> QRDDFHWEEYLKETGSISAPSECFRQSQIPPVNDF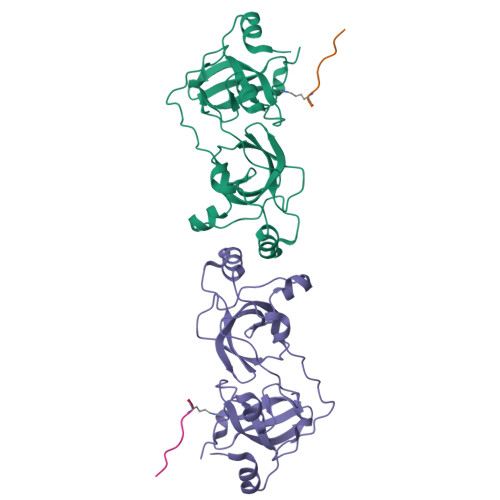KVGMKLEARDPRNATSVCIATVIGITGARLRLRLDGSDNRNDFWRLVDSPDIQPVGTCEKEGDLLQPPLGYQMNTSSWPMFLLETLNGSEMASATLFKKEPPKPPLNNFKVGMKLEAIDKKNPYLICPATIGDVKGDEVHITFDGWSGAFDYWCKYDSRDIFPAGWCRLTGDVLQPPGTS;> VHRLLRKGNYAERVGA> MTENIISVDHLTYQYDENQAPALTDVSFTVHAGEWLAIVGHNGSGKSTLAKSLDGLLPFTQGSVTVGGITLTPETVWQVREQIGMIFQNPDNQFVGATVEDDVAFGLENRQISRDEMVPRVQAALAQVGMTSFAQREPSSLSGGQKQRVALAGIVAIAPKILILDEATSMLDPQGRIEMLAIVRQLRQQQNLTVISITHDIDEAASADRVLVIDDGRLVDEAVPSQ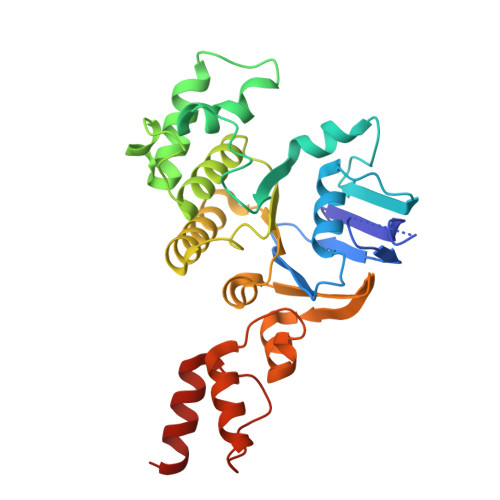IFERGTQLVEMGLDLPFTEKLKAALRQRGITPPTTYQTAAEMEEWLWQSLSNT> GMGSMSTPAASANGGQVLLLPFPAAQGH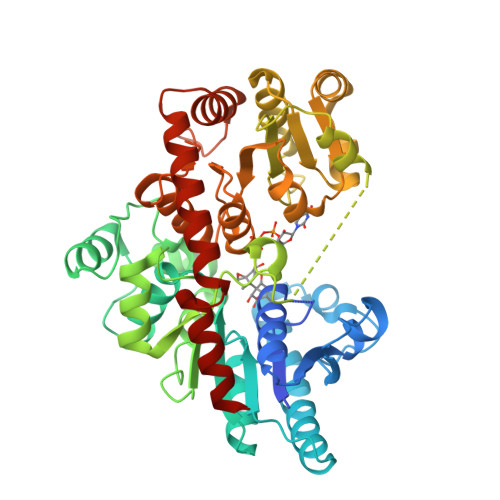TNPMLQFGRRLAYHGLRPTLVTTRYVLSTTPPPGDPFRVAAISDGFDDASGMAALPDPGEYLRTLEAHGARTLAELLLSEARAGRPARVLVYDPHLPWARRVARAAGVATAAFLSQPCAVDLIYGEVCARRLALPVTPTDARGLYARGVLGVELGPDDVPPFVAAPELTPAFCEQSIEQFAGLEDDDDVLVNSFSDLEPKEAAYMESTWRAKTIGPSLPSFYLDDGRLRSNTAYGFNLFRSTVPCMEWLDKQPPRSVVLVSYGTVSTFDVAKLEELGNGLCNSGKPFLWVVRSNEEHKLSVQLRKKCEKRGLIVPFCPQLEVLAHKATGCFLSHCGWNSTLEAIVNGVPLVAMPHWADQPTISKYVESLWGMGVRVQLDKSGILQREEVERCIREVMDGDRKEDYRRNATRLMKKAKESMQEGGSSDKNIAEFAAKYSN(4R,5S)-3-[(2R)-2-{(2S,2'R,4S,5S,5'R)-2,5'-diethyl-5'-[(1S)-1-hydroxyethyl]-4-methyloctahydro-2,2'-bifuran-5-yl}butanoyl]-4-methyl-5-phenyl-1,3-oxazolidin-2-one | C29 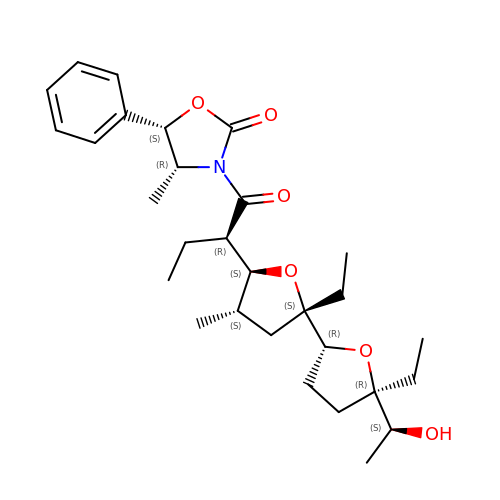H43 N O6 | SYWOXCFBKCIFEM-VTYWIBJUSA-N>HHHHHHGSEKWTSTAIITQPDVGQIAGYNNAMNVIYGQAAPKVSDLQETLIGRFSSAFSALAETLDNQEEPEKLTIEPSVKNQQLPLTVSYVGQTAEGAQMKLAQYIQQVDDKVNQELERDLKDNIA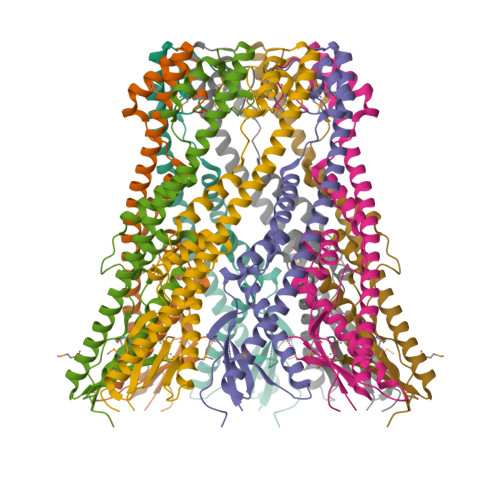LGRKNLQDSLRTQEVVAQEQKDLRIRQIEEALRYADEAKITQPQIQQTQDVTQDTMFLLGSDALKSMIQNEATRPLAFSPAYYQTKQTLLDIKNLKVTADTVHVYRYVMKPTLPVRRDSPK[2x]> MSLALNPAVAPIKSIEFIPVNYQASNWSQNTVVVKVTDENGVYGLGEADGSPDAILAYANIETEHKWLTNITEKAIGRLPIEINAIWDAMYDATQWQGMRGLGMFALSGIDMALYDLAG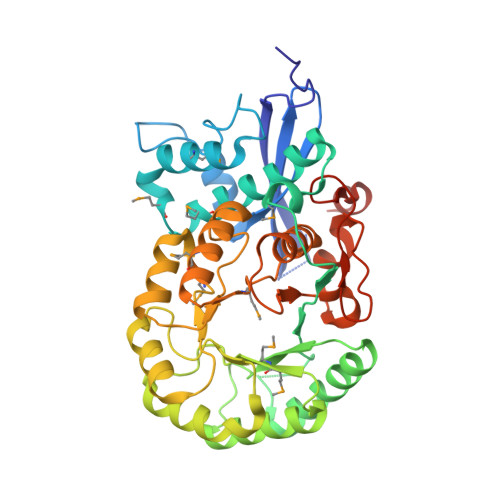KQLGVPAYQLLGGTNKDKVHPYLTLYPAIPVDASLDVAIKGYAPLLEKAKAHNIRAVKVCVPIKADWSTKEVAYYLRELRGILGHDTDMMVDYLYRFTDWYEVARLLNSIEDLELYFAEATLQHDDLSGHAKLVENTRSRICGAEMSTTRFEAEEWITKGKVHLLQSDYNRCGGLTELRRITEMATANNVQVMPHNWKTGITSAAAIHYQFAVGNAPYFEYVHPEFCDGELRKYLVTPEAELVDGGFAKPTAPGLGIDLNQEFLASLEGHHHHHH D-MANNONIC ACID | C6 H12 O7 | 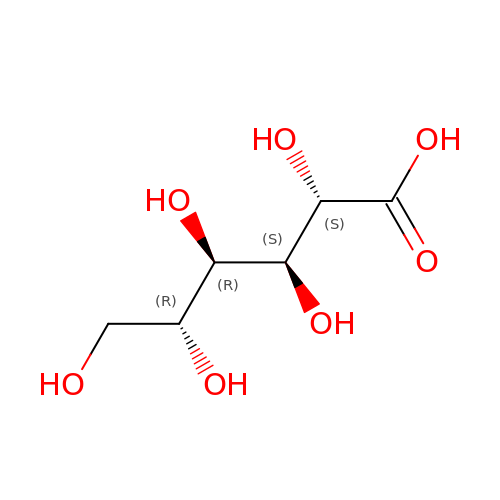RGHNJXZEOKUKBD-MBMOQRBOSA-N(3~{E})-3-[(~{E})-3-oxidanylprop-2-enoyl]iminopropanoic acid | C6 H7 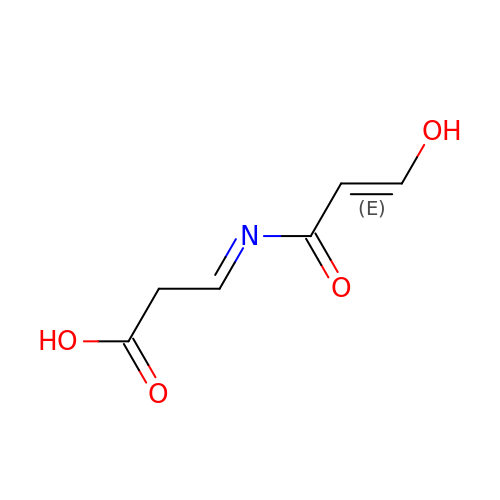N O4 | FVWUPCWGBLBUEE-JKEDICHKSA-N>TPATQPLINAEPAVAAQTEQNPQVGQVMPGVQGADAPVVAQNGPSRDVKLTFAQIAPPPGSMVLRGINPNGSIEFGMRSDEVVTKAMLNLEYTPSPSLLPVQSQLKVYLNDELMGVLPVTKEQLGKKTLAQMPINPLFITDFNRVRLEFVGHYQDVCENPASTTLWLDVGRSSGLDLTYQTLNVKNDLSHFPVPFFDPRDNRTNTLPMVFAGAPDVGLQQASAIVASWFGSRSGWRGQNFPVLYNQLPDRNAIVFATNDKRPDFLRDHPAVKAPVIEMINHPQNPYVKLLVVFGRDDKDLLQAAKGIAQGNILFRGESVVVNEVKPLLPRKPYDAPNWVRTDRPVTFGELKTYEEQLQSSGLEPAAINVSLNLPPDLYLMRSTGIDMDINYRYTMPPVKDSSRMDISLNNQFLQSFNLSSKQEANRLLLRIPVLQGLLDGKTDVSIPALKLGATNQLRFDFEYMNPMPGGSVDNCITFQPVQNHVVIGDDSTIDFSKYYHFIPMPDLRAFANAGFPFSRMADLSQTITVMPKAPNEAQMETLLNTVGFIGAQTGFPAINLTVTDDGSTIQGKDADIMIIGGIPDKLKDDKQIDLLVQATESWVKTPMRQTPFPGIVPDESDRAAETRSTLTSSGAMAAVIGFQSPYNDQRSVIALLADSPRGYEMLNDAVNDSGKRATMFGSVAVIRESGINSLRVGDVYYVGHLPWFERLWYALANHPILLAVLAAISVILLAWVLWRLLRI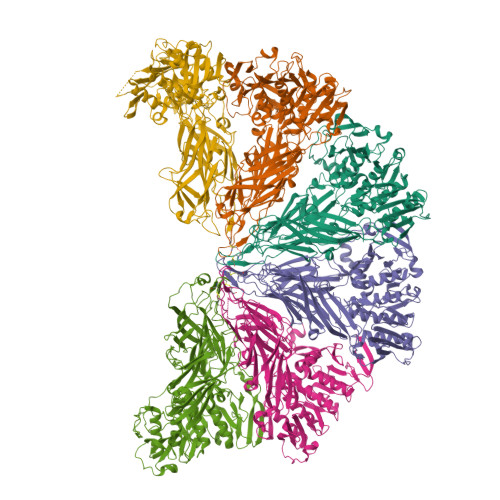ISRRRLNPDNE[6x]>MLIDTHVHLNDEQYDDDLSEVITRAREAGVDRMFVVGFNKSTIERAMKLIDEYDFLYGIIGWHPVDAIDFTEEHLEWIESLAQHPKVIGIGEMGLDYHWDKSPADVQKEVFRKQIALAKRLKLPIIIHNREATQDCIDILLEEHAEEVGGIMHSFSGSPEIADIVTNKLNFYISLGGPVTFKNAKQPKEVAKHVSMERLLVETDAPYLSPHPYRGKRNEPARVTLVAEQIAELKGLSYEEVCEQTTKNAEKLFNL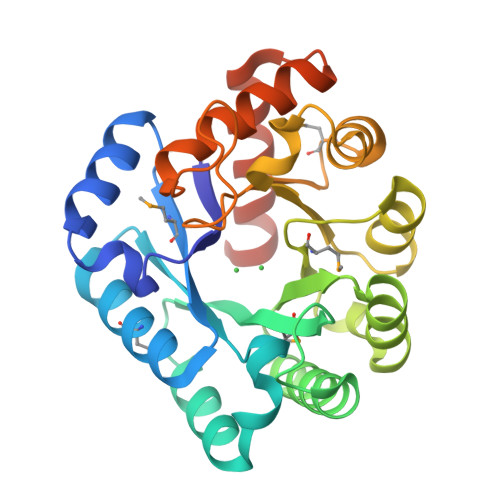NSLEHHHHHH[2x]Ribosome associated complex (RAC), an obligate heterodimer of HSP40 and HSP70 (Zuo1 and Ssz1 in yeast), is conserved in eukaryotes and functions as co-chaperone for another HSP70 (Ssb1/2 in yeast) to facilitate co-translational folding of nascent polypeptides. On the other hand, low-resolution cryo-EM structures of the 80S-RAC complexes and biochemical characterization have identified the contact sites of RAC near the PTE of the ribosome, and more importantly demonstrated the separate binding of the C- and N-terminal parts of Zuo1 to the 40S and 60S subunits, respectively. Structural analyses indicate that RAC on the nascent-chain-free ribosome is in an autoinhibited conformation, and in the presence of a nascent chain at the peptide tunnel exit (PTE), RAC undergoes large-scale structural remodeling to make Zuo1 J-Domain more accessible to Ssb. Our data also suggest a role of Zuo1 in orienting Ssb-SBD proximal to the PTE for easy capture of the substrate.

The best resolved class C2 enabled us to generate a reliable model for both Zuo1 and Ssz1, based on the crystal structure of CtSsz1-NDZuo1 complex34 and the AlphaFold2 predicted model of ScSsz145. Except for a disordered region of Zuo1 (residues 50–70) and a highly flexible β-hairpin of Ssz1 (residues 458–488), the cryo-EM map has well resolved densities for all rest parts of Zuo1-NTD and Ssz1. In this specific conformation, in addition to the previously characterized interactions of Zuo1 ND with Ssz1, two new inter-molecular contact sites were identified. The first involves the first helix of Zuo1 ND (residues 33–44), which is sandwiched between the HPD-containing helix of Zuo1 JD and the IA subdomain of Ssz1 NBD. The second is between the surface of Ssz1 SBD (R521, K534) with the N-terminal sequence of Zuo1 JD (E83, D89), through polar interactions. Very importantly, this conformation of Ssz1 is stabilized by a previously unrecognized interaction of a sequence on the IIB subdomain of Ssz1 NBD with uL24 and the H7-loop of the 25S rRNA. Specifically, H293 of Ssz1 stacks with the base of G85 in H7-loop; S282 and D284 of Ssz1 establish charged interactions with H110 of uL24. Upon this interaction, the H7-loop is seen to undergo a conformation change, being pushed away from the H7:uL24 interface. Secondly, in the State C2 of the RNC-RAC complex, Ssz1 undergoes a very large rotation to flip to the opposite side of Zuo1. In this conformation, Ssz1 sits exactly above the PTE, placing its SBD close to the exit.

> MFSLPTLTSDITVEVNSSATKTPFVRRPVEPVGKFFLQHAQRTLRNHTWSEFERIEAEKNVKTVDESNVDPDELLFDTELADEDLLTHDARDWKTADLYAAMGLSKLRFRATESQIIKAHRKQVVKYHPDKQSAAGGSLDQDGFFKIIQKAFETLTDSNKRAQYDSCDFVADVPPPKKGTDYDFYEAWGPVFEAEARFSKKTPIPSLGNKDSSKKEVEQFYAFWHRFDSWRTFEFLDEDVPDDSSNRDHKRYIERKNKAARDKKKTADNARLVKLVERAVSEDPRIKMFKEEEKKEKERRKWEREAGARAEAEAKAKAEAEAKAKAESEAKANASAKADKKKAKEAAKAAKKKNKRAIRNSAKEADYFGDADKATTIDEQVGLIVDSLNDEELVSTADKIKANAAGAKEVLKESAKTIVDSGKLPSSLLSYFV;> MSSPVIGITFGNTSSSIAYINPKNDVDVIANPDGERAIPSALSYVGEDEYHGGQALQQLIRNPKNTIINFRDFIGLPFDKCDVSKCANGAPAVEVDGKVGFVISRGEGKEEKLTVDEVVSRHLNRLKLAAEDYIGSAVKEAVLTVPTNFSEEQKTALKASAAKIGLQIVQFINEPSAALLAHAEQFPFEKDVNVVVADFGGIRSDAAVIAVRNGIFTILATAHDLSLGGDNLDTELVEYFASEFQKKYQANPRKNARSLAKLKANSSITKKTLSNATSATISIDSLADGFDYHASINRMRYELVANKVFAQFSSFVDSVIAKAELDPLDIDAVLLTGGVSFTPKLTTNLEYTLPESVEILGPQNKNASNNPNELAASGAALQARLISDYDADELAEALQPVIVNTPHLKKPIGLIGAKGEFHPVLLAETSFPVQKKLTLKQAKGDFLIGVYEGDHHIEEKTLEPIPKEENAEEDDESEWSDDEPEVVREKLYTLGTKLMELGIKNANGVEIIFNINKDGALRVTARDLKTGNAVKGEL> PLTEQEIDELCDEWVPEPLIPPITEDMKHEPPVLESAAGPHTTVNGKDVVNFASANYLGL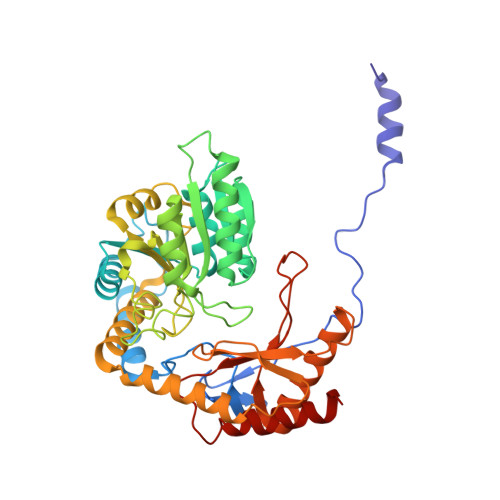IGHEKLLESCTSALEKYGVGSCGPRGFYGTIDVHLDCETRISKFLGTPDSILYSYGLSTMFSTIPCFCKKGDVIVADEGVHWGIQNGLQLSRSTIVYFKHNDMESLRITLEKIMTKYKRSKNLRRYIVAEAVYQNSGQIAPLDEIVKLKEKYRFRVILDESNSFGVLGRSGRGLAEHHSVPIEKIDVVTAAMGHALATEGGFCTGNARIIDYQRLSSSGYVFSASLPPYLASAAITAIDVIDQNPDMLVKLKQNVALLWKGLSDIKGMSLTSNRESPIVFLKLEKSSGSAKDDLLLLEKMADRALKEDSLLVVSSKRSFLDKCRLPVGIKLYVSAGHSESDLLKASESLKRLASELLLKS>[2x]IQTTAPPVKESSFVEKMKKTGRNIIVFYGSQTGTAEEFANRLSKDAHRYGMRGMSADPEEYDLADLSSLPEIDKSLVVFCMATYGEGDPTDNAQDFYDWLQETDVDLTGVKFAVFGLGNKTYEHFNAMGKYVDQRLEQLGAQRIFELGLGDDDGNLEEDFITWREQFWPAVCEFFGVEATGEESSIRQYELVVHEDMDVAKVYTGEMGRLKSYENQKPPFDAKNPFLAAVTANRKLNQGTERHLMHLELDISDSKIRYESGDHVAVYPANDSALVNQIGEILGADLDVIMSLNNLDEESNKKHPFPCPTTYRTALTYYLDITNPPRTNVLYELAQYASEPSEQEHLHKMASSSGEGKELYLSWVVEARRHILAILQDYPSLRP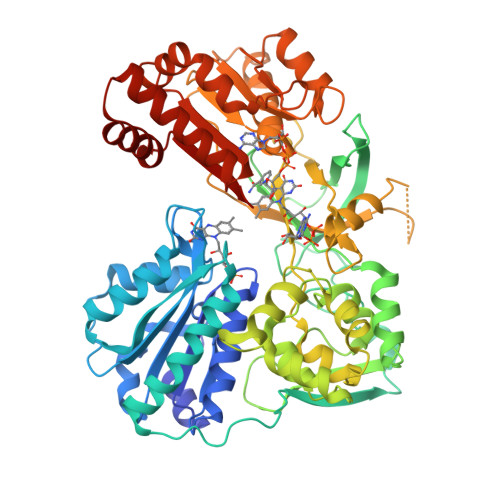PIDHLCELLPRLQARYYSIASSSKVHPNSVHICAVAVEYEAKSGRVNKGVATSWLRAKEPAGENGGRALVPMFVRKSQFRLPFKSTTPVIMVGPGTGIAPFMGFIQERAWLREQGKEVGETLLYYGCRRSDEDYLYREELARFHKDGALTQLNVAFSREQAHKVYVQHLLKRDREHLWKLIHEGGAHIYVCGDARNMAKDVQNTFYDIVAEFGPMEHTQAVDYVKKLMTKGRYSLDVGS>[3x]MPELLNPAPVAHLRHLLRAHSPLVHCMTNDVVQTFTANVLLAVGASPAMVIDPREAAQFAAIADALLINVGTLTEDRAVAMRAAVEHARQAGKPWTLDPVAVGALTVRTAFCHELLALQPAAIRGNASEILALAGMSAGGRGVDTTDTAAAALPAAQALARRLATVVAVTGEVDYVTDGERVLSVAGGNPLMTRVVGTGCALSAVVAASAALPG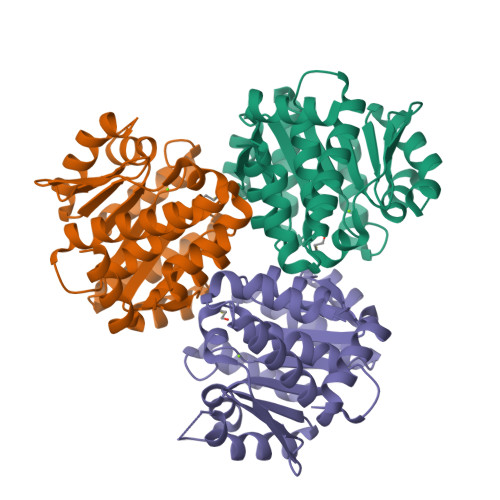DRLENVAAACGLMKQAGEIAARQGGPGSFIPAFLDALYQEVQG>[2x]GNSATSADEQPHIGNYRLLKTIGKGNFAKVKLARHILTGKEVAVKIIDKTQLNSSSLQKLFREVRIMKVLNHPNIVKLFEVIETEKTLYLVMEYASGGEVFDYLVAHGRMKEKEARAKFRQIVSAVQYCHQKFIVHRDLKAENLLLDADMNIKIADFGFSNEFTFGNKLDAFCGAPPYAAPEL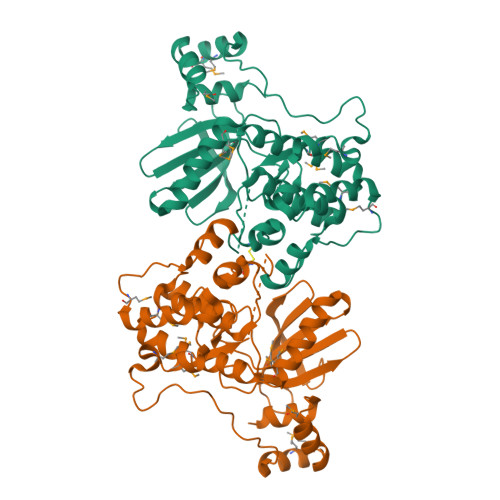FQGKKYDGPEVDVWSLGVILYTLVSGSLPFDGQNLKELRERVLRGKYRIPFYMSTDCENLLKKFLILNPSKRGTLEQIMKDRWMNVGHEDDELKPYVEPLPDYKDPRRTELMVSMGYTREEIQDSLVGQRYNEVMATYLLLGYK>[5x]MGSSHHHHHHSQDPLVPRGSWETEERPRTREEECHFYAGGQVYPGEASRVSVADHSLHLSKAKISKPAPYWEGTAVIDGEFKELKL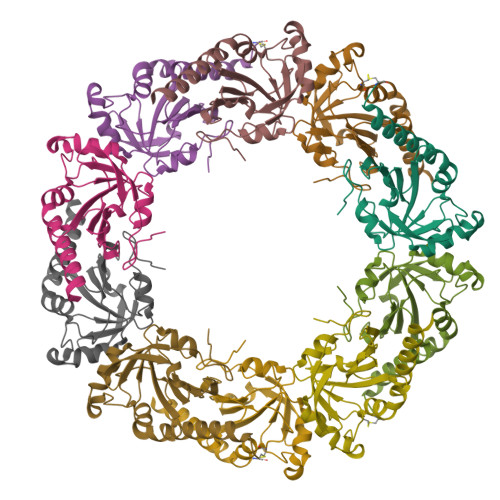TDYRGKYLVFFFYPLDFTFVCPTEIIAFGDRLEEFRSINTEVVACSVDSQFTHLAWINTPRRQGGLGPIRIPLLSDLTHQISKDYGVYLEDSGHTLRGLFIIDDKGILRQITLNDLPVGRSVDETLRLVQAFQYTDKHGEVCPAGWKPGSETIIPDPAGKLKYFDKLN>[2x]MASVNSLEKHSWYHGPVSRNAAEYLLSSGINGSFLVRESESSPGQRSISLRYEGRVYHYRINTASDGKLYVSSESRFNTLAELVHHHST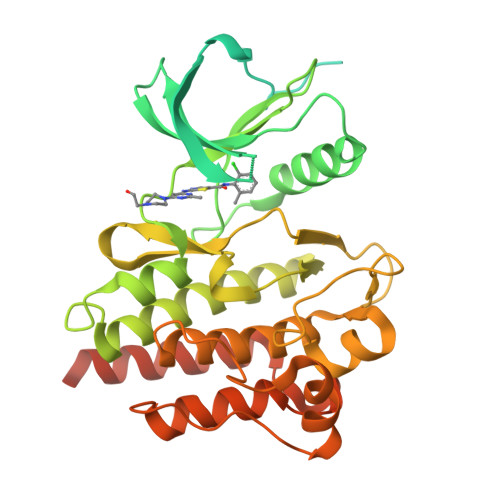VADGLITTLHYPAPKRNKPTVYGVSPNYDKWEMERTDITMKHKLGGGQYGEVYEGVWKKYSLTVAVKTLKEDTMEVEEFLKEAAVMKEIKHPNLVQLLGVCTREPPFYIITEFMTYGNLLDYLRECNRQEVNAVVLLYMATQISSAMEYLEKKNFIHRDLAARNCLVGENHLVKVADFGLSRLMTGDTYTAHAGAKFPIKWTAPESLAYNKFSIKSDVWAFGVLLWEIATYGMSPYPGIDLSQVYELLEKDYRMERPEGCPEKVYELMRACWQWNPSDRPSFAEIHQAFETMFQESSISDEVEKELGKQGVLEHHHHHH>[2x]SSPVAQKYDYILVGGGTAACVLANRLSADGSKRVLVLEAGPDNTSRDVKIPAAITRLFRSPLDWNLFSELQEQLAERQIYMARGRLLGGSSATNATLYHRGAAGDYDAWGVEGWSSEDVLSWFVQAETNADFGPGAYHGSGGPMRVENPRYTNKQLHTAFFKAAEEVGLTPNSDFNDWSHDHAGYGTFQVMQDKGTRADMYRQYLKPVLGRRNLQVLTGAAVTKVNIDQAAGKAQALGVEFSTDGPTGERLSAEL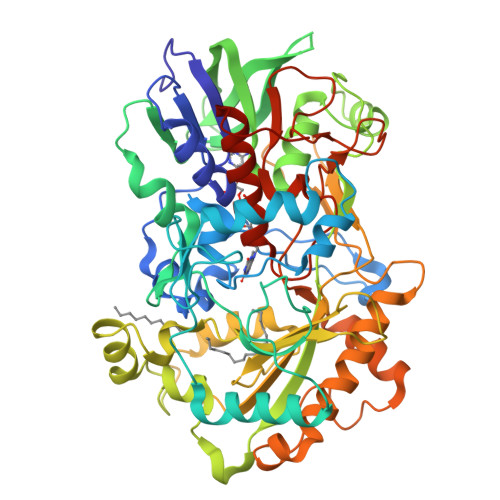APGGEVIMCAGAVHTPFLLKHSGVGPSAELKEFGIPVVSNLAGVGQNLQDQPACLTAAPVKEKYDGIAISDHIYNEKGQIRKRAIASYLLGGRGGLTSTGCDRGAFVRTAGQALPDLQVRFVPGMALDPDGVSTYVRFAKFQSQGLKWPSGITMQLIACRPQSTGSVGLKSADPFAPPKLSPGYLTDKDGADLATLRKGIHWARDVARSSALSEYLDGELFPGSGVVSDDQIDEYIRRSIHSSNAITGTCKMGNAGDSSSVVDNQLRVHGVEGLRVVDASVVPKIPGGQTGAPVVMIAERAAALLTGKATIGASAAAPATVAA>[2x]WTNTSGSCRGRCFERTFSNCRCDAACVSLGNCCLDFQETCVEPTHIWTCNKFRCGEKRLSRFVCSCADDCKTHNDCCINYSSVCQDKKSWVEETCESIDTPECPAEFESPPTLLFSLDGFRAEYLHTWGGLLPVISKLKNCGTYTKNMRPMYPTKTFPNHYSIVTGLYPESHGIIDNKMYDPKMNASFSLKSKEKFNPLWYKGQPIWVTANHQEVKSGTYFWPGSDVEIDGILPDIYKVYNGSVPFEERILAVLEWLQLPSHERPHFYTLYLEEPDSSGHSHGPVSSEVIKALQKVDRLVGMLMDGLKDLGLDKCLNLILISDHGMEQGSCKKYVYLNKYLGDVNNVKVVYGPAARLRPTDVPETYYSFNYEALAKNLSCREPNQH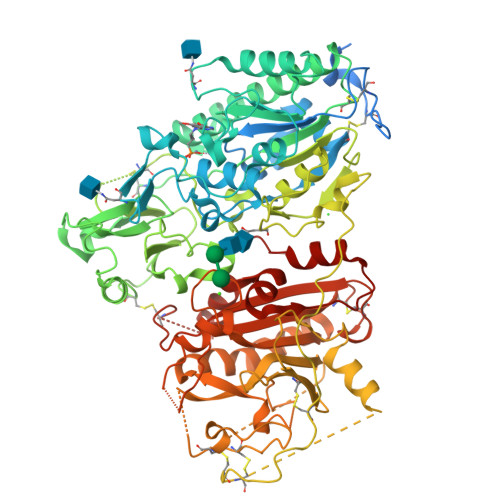FRPYLKPFLPKRLHFAKSDRIEPLTFYLDPQWQLALNPSERKYCGSGFHGSDNLFSNMQALFIGYGPAFKHGAEVDSFENIEVYNLMCDLLGLIPAPNNGSHGSLNHLLKKPIYNPSHPKEEGFLSQCPIKSTSNDLGCTCDPWIVPIKDFEKQLNLTTEDDDIYHMTVPYGRPRILLKQHRVCLLQQQQFLTGYSLDLLMPLWASYTFLSNDQFSRDDFSNCLYQDLRIPLSPVHKCSYYKSNSKLSYGFLTPPRLNRVSNHIYSEALLTSNIVPMYQSFQVIWHYLHDTLLQRYAHERNGINVVSGPVFDFDYDGRYDSLEILKQNSRVIRSQEILIPTHFFIVLTSCKQLSETPLECSALESSAYILPHRPDNIESCTHGKRESSWVEELLTLHRARVTDVELITGLSFYQDRQESVSELLRLKTHLPIFSQED>MAQRLDGARFRYLNEQLY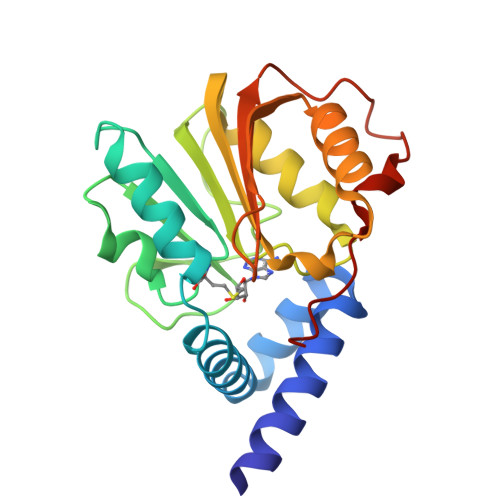SGPSSAAQRLFQEDPEAFLLYHRGFQSQVKKWPLQPVDRIARDLRQRPASLVVADFGCGDCRLASSIRNPVHCFDLASLDPRVTVCDMAQVPLEDESVDVAVFCLSLMGTNIRDFLEEANRVLKPGGLLKVAEVSSRFEDVRTFLRAVTKLGFKIVSKDLTNSHFFLFDFQKTGPPLVGPKAQLSGLQLQPCLYKRR[2x]> SMEGMLADFVSQTSPMIPSIVVHCVNEIEQRGLTETGLYRISGCDRTVKELKEK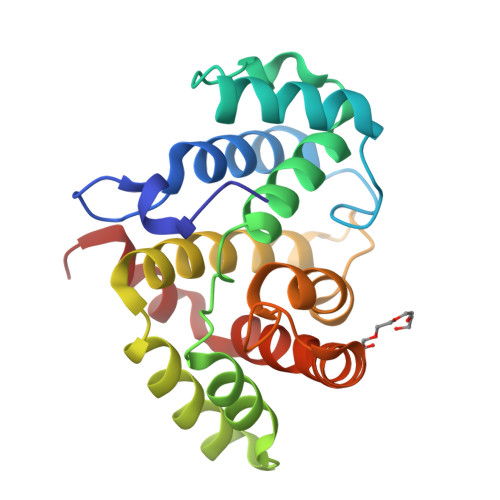FLRVKTVPLLSKVDDIHAICSLLKDFLRNLKEPLLTFRLNRAFMEAAEITDEDNSIAAMYQAVGELPQANRDTLAFLMIHLQRVAQSPHTKMDVANLAKVFGPTIVAHAVPNPDPVTMLQDIKRQPKVVERLLSLPLEYWSQFMMVE> MYAPAAEDEHTITNWSGTHAVRPKRFFQPESVEELEKIVKEAHEKGQKIRPVGSGLSPNGLAFSEDGMVSLALMDKVLHVDKEKKQVTVQAGARVQQVVDALRPHGLTLQNFASISEQQIGGFIQVGAHGTGARIPPVDEQVVSMKLVTPAKGTIELSEEKDPELFRLARCGLGALGVVTEVTLQCVPRHKLLEHTFVATMKEVKKNHEKLLRENKHVRYMWIPYTDTVVVVTCNPLPEGKKAPKVKPQYSEDEKLQPLRNLLREAAPPARAPEVAAPSSSETSPEVSGLSFTELRDALLAVDPLDTEWVKRVNQAEAEFWKRSEGYRVGWSDEILGFDCGGQQWVSEVAFPAGTLEKPSAADLEYMEELMRLINKEGIPAPAPIEQRWTAGSSSPMSPAYSPSPDSVFSWVNIIMYLPTEDEEQRKAITEAFRQYRKLCETRLWDKYGAAEHWAKIEVPEDPEELEALRERLRKRYPGVDKFNKARRELDPKNILSNDMIDSLFPAAESA

In photosynthetic organisms, L-ascorbic acid is produced in the Smirnoff-Wheeler pathway by the multi-step conversion of D-mannose-6-phosphate to L-galactono-1,4-lactone, the substrate for the final biosynthetic enzyme, L-galactono-1,4-lactone dehydrogenase (GalDH) [EC 1.3.2.3]9,15. GULO, ALO, and GalDH are generally named aldonolactone oxidoreductases and form a group of sequence-related flavoenzymes belonging to the vanillyl-alcohol oxidase family. They oxidize the C2 carbon atom of their monosaccharide substrates and thereby generate the characteristic, redox-reactive C2-C3 double bond of L-ascorbic acid and its analogs. GalDH is a dehydrogenase that reacts poorly with oxygen.

The structural comparison shows that the only conspicuous change between the substrate-binding sites of the two enzymes is the replacement of Gly413 in GalDH to Asn363 in GULO (residue numbers refer to vGalDH and mGULO). We sought to unveil the role of this amino acid exchange by introducing the G413N mutation in wild-type and A113G GalDHs. Encouragingly, however, we found that the single G413N mutants had sustained activities. Both G413N sGalDH and vGalDH displayed a selective decrease in the KM for L-gulono-1,4-lactone and no drastic alterations in the KM for L-galactono-1,4-lactone or the respective kcat values. We further performed the crystallographic analysis of G413N vGalDH at 2.3 Å resolution using crystals that were soaked in a solution comprising L-gulono-1,4-lactone. The B-factors of the bound sugar were notably high. However, despite this, the electron density was of sufficient quality to conclude that the conformation and orientation of L-gulono-1,4-lactone are highly similar to that of L-galactono-1,4-lactone bound to the wild-type enzyme, with the obvious exception of the 3-hydroxyl group position. The substrate-binding environment is likewise mostly retained in the mutant structure. The only differences affect Glu386, which shifts towards Arg219 and no longer forms an H-bond with the ligand, and the newly formed H-bond between the ligand O3 and Arg388. The carbamide group of the introduced Asn413 is nestled on the sugar ring and in van der Waals contact with the substrate O3. Collectively, these data demonstrate that the GalDH versus GULO distinction can be primarily explained by very few amino acid changes in an otherwise remarkably well-conserved catalytic cavity.> EKPAAVVA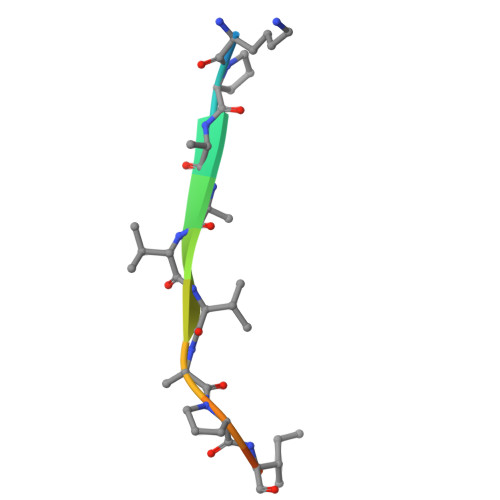PITTG> CACGAGCCTGAT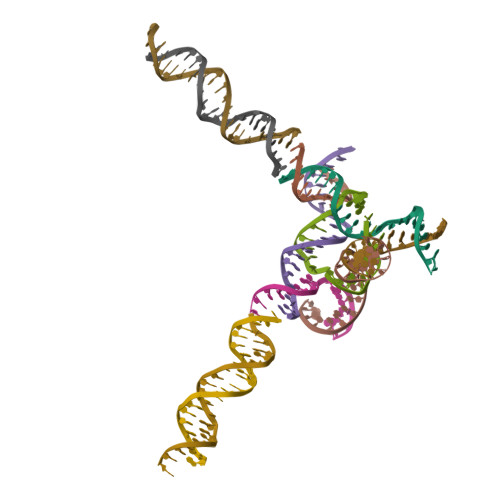CGGACAAGA;> AGGCAGCCTGTACGGACATCA;> AACCTACCTGGCAGGACGACT;> GATCTTGTGGCTGC;> TTAGTCGTGGCTCG;> ACTGATGTGGTAGG;> TCACCTGCCACCGTACACCGA;> TGCTAGGCTAACTCGCTAGCG;> TCCGCTAGCGAGTTAGCCTAG;> GTCTCTGCTAGATCGTCAGCA;> CTTGCTGACGATCTAGCAGAG>[2x]MGHHHHHHEDRDPTQFEERHLKFLQQLGKGNFGSVEMCRYDPLQDNTGEVVAVK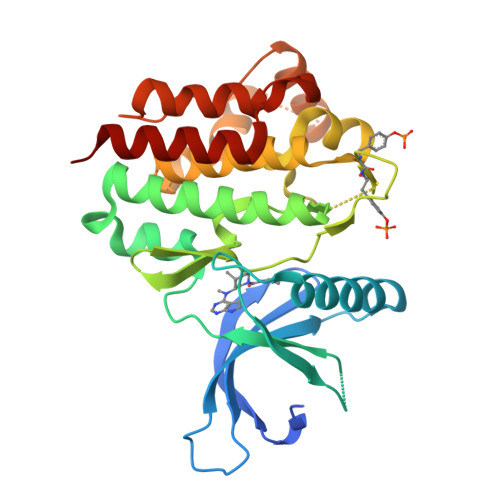KLQHSTEEHLRDFEREIEILKSLQHDNIVKYKGVCYSAGRRNLKLIMEYLPYGSLRDYLQKHKERIDHIKLLQYTSQICKGMEYLGTKRYIHRDLATRNILVENENRVKIGDFGLTKVLPQDKEYYKVKEPGESPIFWYAPESLTESKFSVASDVWSFGVVLYELFTYIEKSKSPPAEFMRMIGNDKQGQSIVTHLIELLKNNGRLPRPDGCPDEIYMIMTECWNNNVNQRPSFRDLALRVDQIRDNMAG> MATLQDIGVSAGINILSAFVFFIIFAVLRLQPFNDRVYFSKWYLKGLRSSPARGGAFAQRFVNLDFRSYMKFLNWMPEALKMPEPELIDHAGLDSVVYLRIYWLGLKIFTPIAVLAWAVLVPVNWTNNTLEMAKQLRNVTSSDIDKLSVSNIPEYSMRFWTHIVMAYAFTIWTCYVLMKEYETIANMRLQFVASEARRPDQFTVLVRNVPPDADESVSELVEHFFLVNHPDHYLTHQVVCNANKLADLVKKKKKLQNWLDYYQLKYARNNSQRIMVKLGFLGLWGQKVDAIEHYIAEIDKISKEISKEREEVVNDPKAIMPAAFVSFKTRWAAAWCAQTQQTRNPTQWLTEWAPEPRDVFWSNLAIPYVSLTVRRLIMHVAFFFLTFFFIVPIAFVQSLATIEGIVKAAPFLKFIVDDKFMKSVIQGFLPGIALKLFLAFLPSILMIMSKFEGFTSISSLERRAAFRYYIFNLVNVFLASVIAGAAFEQLNSFLNQSANQIPKTIGVAIPMKATFFITYIMVDGWAGVAGEILMLKPLIMFH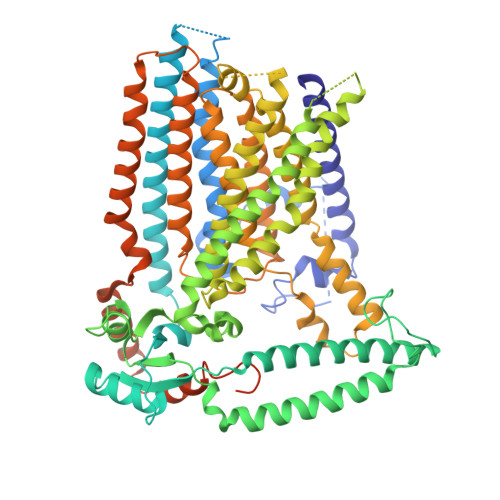LKNAFLVKTDKDREEAMDPGSIGFNTGEPRIQLYFLLGLVYAPVTPMLLPFILVFFALAYIVYRHQIINVYNQEYESAAAFWPDVHGRVIAALVISQLLLMGLLGTKHAALAAPFLIALPVLTIGFHHFCKGRYEPAFIRYPLQEAMMKDTLETAREPNLNLKGYLQNAYVHPVFKGDEDDYDIDDKLGKFEDEAIIVPTKRQSRRNTPAPSIISGDDSPSLPFSGKLVSNSLEV>[2x]MQGVNIYNISAGTSVDLAAPVTTGDIVTFFSSALNLNAGAGNPNN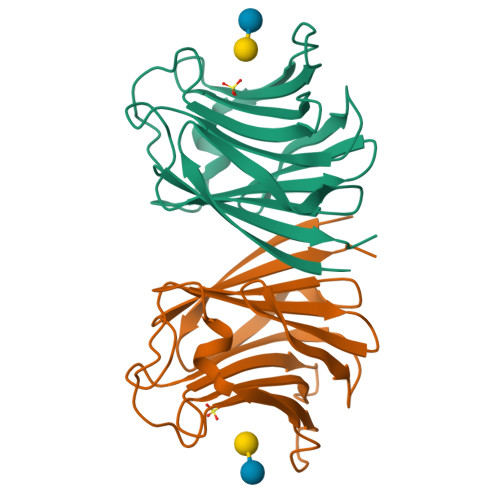TTLNLFAENGAYLLHIAFRLQENVIIFNSRQPDGPWLVEQRVSDVANQFAGIDGKAMVTVFDHGDKYQVVINEKTVIQYTKQISGLTSSLSYNATEETSIFSTVVEAVTYTGLALEHHHHHH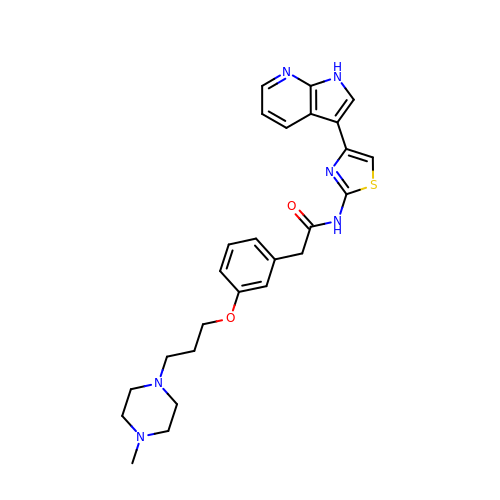2-[3-[3-(4-methylpiperazin-1-yl)propoxy]phenyl]-~{N}-[4-(1~{H}-pyrrolo[2,3-b]pyridin-3-yl)-1,3-thiazol-2-yl]ethanamide | C26 H30 N6 O2 S | KWQRIWDMNAKJAF-UHFFFAOYSA-N>MSMRDAVICEPVRTPIGRYGGMFRSLTAVDLGVTALKGLLERTGIAADQVEDVILGHCYPNSEAPAIGRVVALDAGLPITVPGMQVDRRCGSGLQAVIQACLQVRSGDHDLVVAGGAESMSNVAFYSTDMRWGGARTGVQIHDGLARGRTTAGGKFHPVPGGMLETAENLRREYHISRTEQDELAVRSHQRAVAAQSEGVLAEEIIPVPVRTRDGEETISVDEHPRADTTVEALAKLKPVLLKQDPEATVTAGNSSGQNDAASMCIVTTPEKAAELGLKPLVRLVSWGSAGVAPDLMGIGPVPATEVALAKAG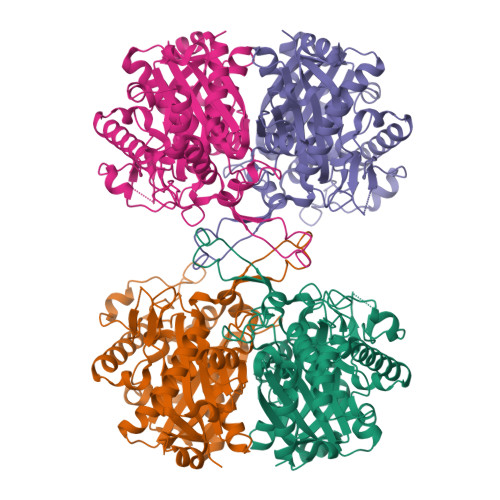LTLADIDLIELNEAFAAQALAVMREWKFGEADHERTNVRGSGISLGHPVGATGGRMLATLARELHRREARYGLETMCIGGGQGLAAVFERVQEG[12x]>PMFIVNTNVPRASVPDGFLSELTQQLAQATGKPPQYIAVHVVPDQGMAFGGSSEPCALCSLHSIGKIGGAQNRSYSKLLCGLLAERLRISPDRVYINYYDMNAANVGWNNSTFA[3x]

Macrophage Migration Inhibitory Factor (MIF) is a ubiquitous multifunctional protein and a key player in the inflammatory response and innate immunity. MIF has two enzymatic activities: an evolutionarily well conserved keto-enol tautomerase activity and a thiol-protein oxido-reductase activity that is mediated by the C56ALC59 motif. X-ray structural studies have consistently shown that MIF exists as a homotrimer. Each MIF monomer consists of 114 amino acids and is composed of two anti-parallel α-helices packed against a four-stranded β-sheet.

To elucidate the role of intersubunit interactions involving Leu46 on the structure and stability of MIF, we compared the structural stability, and biophysical properties of wt, L46A, L46F and L46G mutants at the secondary, tertiary and quaternary structure levels. To understand the role of Leu46 mutations on the three-dimensional structure of MIF, we also determined the crystal structures of L46F, L46A and L46G huMIF at 1.70 Å, 1.70 Å and 1.60 Å, respectively. Similar to the wild type species, Leu46 mutants crystallized as homotrimeric proteins with dimensions of approximately 35 Å×50 Å×50 Å. In agreement with our previous structural studies, X-ray crystal structures of MIF variants demonstrate that the Leu46 mutants conserve the same three-dimensional structure pattern as the wt protein. Static light scattering, in agreement with the analytical ultracentrifugation data, demonstrated that wt, L46F, L46A and L46G exist as stable trimers. Finally, crystallographic data and enzymatic assays do not show any drastic conformational change of the catalytic site or activity of MIF upon Leu46 mutations. Using hydroxyphenylpyruvate as a substrate, we showed that all Leu46 mutants are enzymatically active. In our case, chemical shift measurements demonstrate an extremely high similarity between L46A and L46G huMIF, whereas the L46F mutant exhibits a slightly different chemical shift pattern. Thus, decreasing the hydrophobicity of residue 46 (via mutations L46A and L46G) destabilizes the hydrophobic pocket and results in distant structural perturbation that is transmitted through the backbone, affecting the tertiary structure of the MIF. Taken together, our data suggest that the intersubunit interactions involving the residue Leu46 play a key role in the structural stability of MIF and provide new insights into the role of a novel intersubunit hydrophobic pocket in modulating MIF’s conformation, stability, and potentially its receptor binding and biological activity.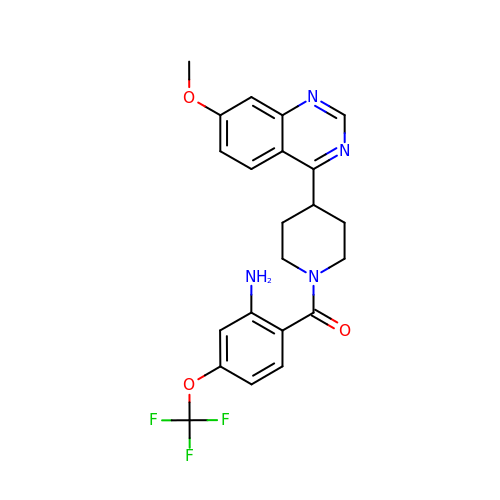[2-azanyl-4-(trifluoromethyloxy)phenyl]-[4-(7-methoxyquinazolin-4-yl)piperidin-1-yl]methanone | C22 H21 F3 N4 O3 | UCMVZMXGBOBQEZ-UHFFFAOYSA-N(~{E})-3-[2-(dihydroxyboranyl)phenyl]prop-2-enoic 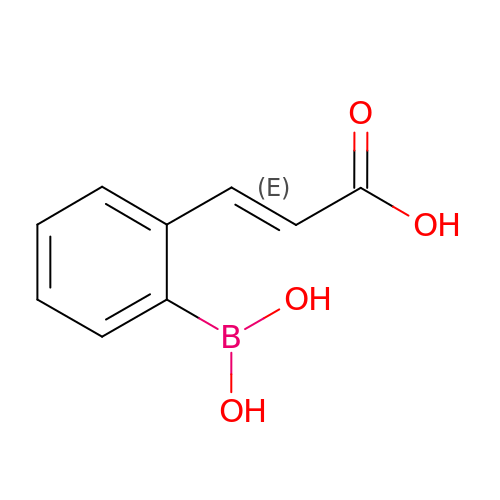acid | C9 H9 B O4 | OPFDGNUJQALQFL-AATRIKPKSA-N> GSMKGSRIELGDVTPHNIKQLKRLNQVIFPVSYNDKFYKDVLEVGELAKLAYFNDIAVGAVCCRVDHSQNQKRLYIMTLGCLAPYRRLGIGTKMLNHVLNICEKDGTFDNIYLHVQISNESAIDFYRKFGFEIIETKKNYYKRIEP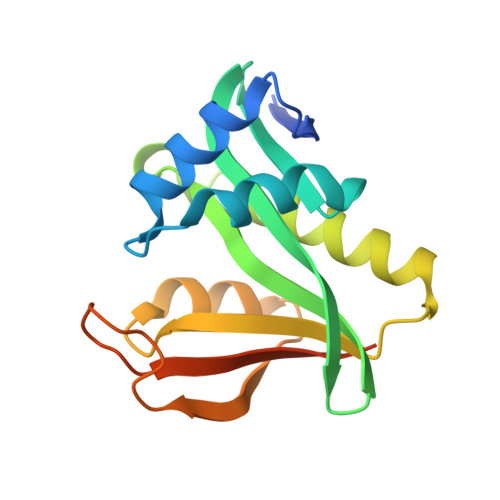ADAHVLQKNLKVPSGQNADVQKTDN> VKGQGRGCLLKEIHLNVTDLDLG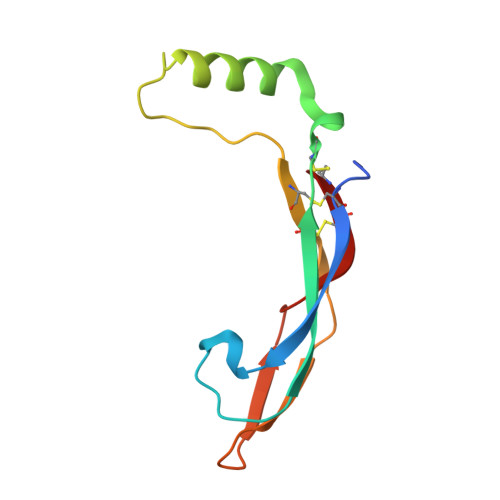YRTKEELIFRYCSGPCHDAETNYDKILNNLTHNKKLDKDTPSRTCCRPIAFDDDISFLDDSLEYHTLKKHSAKKCACV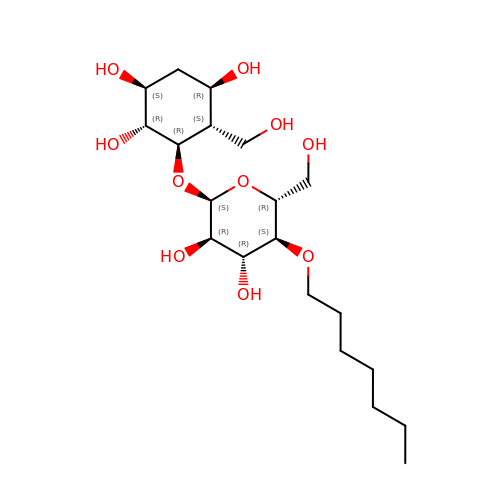(1~{R},2~{S},4~{R},5~{S},6~{R})-6-[(2~{S},3~{R},4~{R},5~{S},6~{R})-5-heptoxy-6-(hydroxymethyl)-3,4-bis(oxidanyl)oxan-2-yl]oxy-5-(hydroxymethyl)cyclohexane-1,2,4-triol | C20 H38 O10 | JXHBWOMWKSCDSB-ZXVXKJDSSA-N> NIPRVRNVLFSSQVMYDNAQLATRDYSLVMR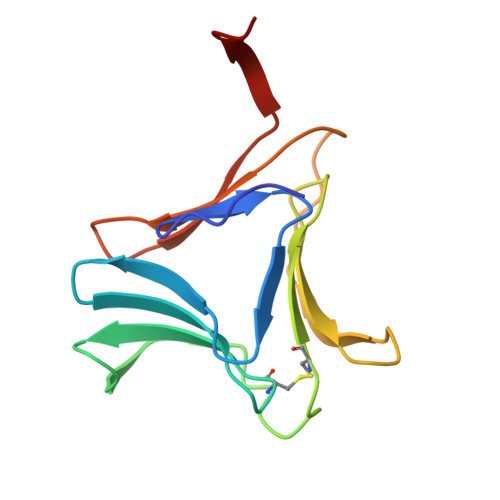DDCNLVLTKGSKTNIVWESGTSGRGQHCFMRLGHSGELDITDDRLNTVFVSNTVGQEGDYVLILQINGQAVVYGPAVWSTAA> MQTLSERLKKRRIALKMTQTELATKAGVKQQSIQLIEAGVTKRPRFLFEIAMALNCDP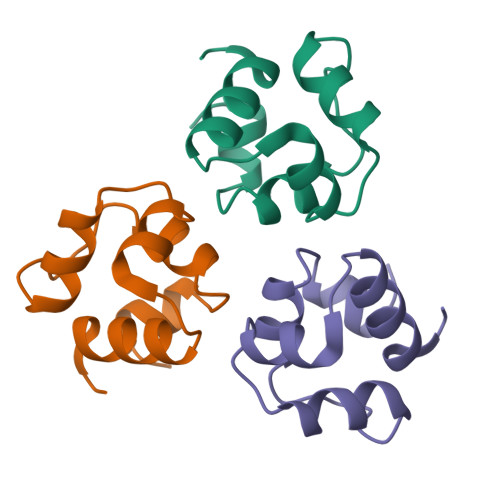VWLQYGTKRGKAA> MDARATIPEHIARTVILPQGYADDEVIYPAFKWLRDEQPLAMAHIEGYDPMWIATKHADVMQIGKQPGLFSNAEGSEILYDQNNEAFMRSISGGCPHVIDSLTSMDPPTHTAYRGLTLNWFQPASIRKLEENIRRIAQASVQRLLDFDGECDFMTDCALYYPLHVVMTALGVPEDDEPLMLKLTQDFFGVHEPDEQAVAAPRQSADEAARRFHETIATFYDYFNGFTVDRRSCPKDDVMSLLANSKLDGNYIDDKYINAYYVAIATAGHDTTSSSSGGAIIGLSRNPEQLALAKSDPALIPRLVDEAVRWTAPVKSFMRTALADTEVRGQNIKRGDRIMLSYPSANRDEEVFSNPDEFDITRFPNRHLGFGWGAHMCLGQHLAKLEMKIFFEELLPK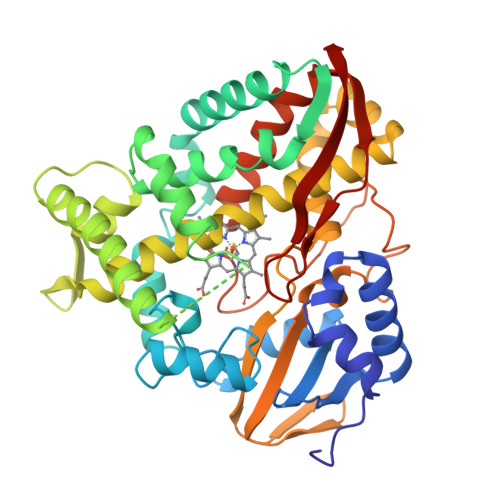LKSVELSGPPRLVATNFVGGPKNVPIRFTKA A common step during their assembly is polyketide trimming, which Afyg1p, Wdyg1p, and PlAntI catalyze. In summary, the N‐ and C‐domains in all three enzymes are oriented in a back‐to‐back fashion forming an interface that encloses the intramolecular binding cavity next to the active site. The catalytic triad is formed exclusively by the α/β‐hydrolase domain with the nucleophilic serine located in the consensus GXSXG esterase motif. The resulting Ser‐His‐Asp network is perfectly aligned with distances in the range of 2.5–2.8 Å between the active‐site residues.

To investigate the specificity pocket and the underlying binding modes of Wdyg1p, conjugated naphthalenes substituted with two hydroxyl‐groups and the product 1,3,6,8‐tetrahydroxynaphthalene (THN) were screened as potential ligands. The ligand is buried at the interface of the N‐ and C‐domain. The 1─OH of 1,3‐DHN is H‐bonded to Glu381Oε (2.3 and 3.5 Å), and the 3─OH interacts with the indole nitrogen of Trp196 (3.1 Å), whereas the planar naphthalene ring system is pi‐stacked between Met379 and Tyr39. Taken together, THN and 1,3‐DHN are located at the edge of Wdyg1p's specificity pocket and facilitate different in‐plane orientations. Thereby, the bottom of the specificity pocket is defined by Glu381 and Trp196, which spans 7 × 12 × 12 Å3.

>MGWSHPQFEKENLYFQGSATEKYYIRDAITKPAVHHESYQKLWETKWKKPCEMGVYPFMFGSIKDFEPVAQEIIKKGLKEPYDWDEYAQMYFPKAEELAKIAEEAEAAGEKEKASEYYLRSSAVYRISRFPTPRSEKQKYAWRKGCEVFYKGAALMEYPIKEVRIPHKHGIEGEGDVVPVNFLLPPNASETSPVPCVLIITGLDGYRTELAVWQQGWRSKGVATVIAEIPGTGDSPALRQDPTSPDRQWSSVLDWIESQKAVDSKKIVAWGFSTGGYYALRMAHTHKDRLLATISLGGGAHHMFDREWLEHANKLEYPFDLSNTLAYKFGYPDLESFIEESSKFSLLNDGTLQKPCTKVLLVNGNDDEIFPIDDMFVSLENGQPKLARMVKGKKHMGEPESFSIILEWIHKLLGLDGKIKEQLAMIPSRTK[2x]> PAKKPLTKIVSHLLVAEPD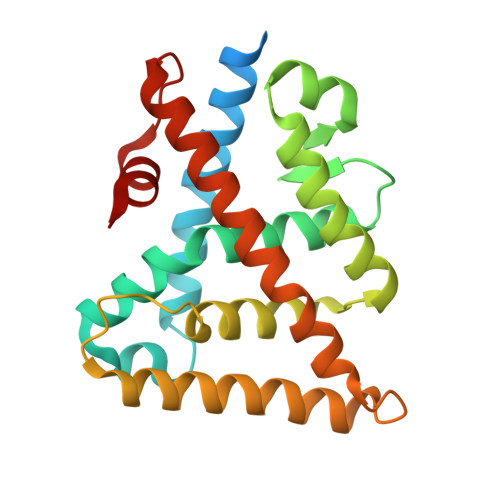KLYAMPPPGMPEGDIKALTTLCDLADRELVVIIGWAKHIPGFSSLSLGDQMSLLQSAWMEILILGIVYRSLPYDDKLVYAEDYIMDEEHSRLAGLLELYRAILQLVRRYKKLKVEKEEFVTLKALALANSDSMHIEDLEAVQKLQDLLHEALQDYELSQHHEEPWRTGKLLLTLPLLRQTAAKAVQHFYSVKLQGKVPMHKLFLEMLEAKV(1S,3R,4R,6S)-1,3,4,6-TETRAPKISPHOSPHATE | C6 H16 O18 P4 | 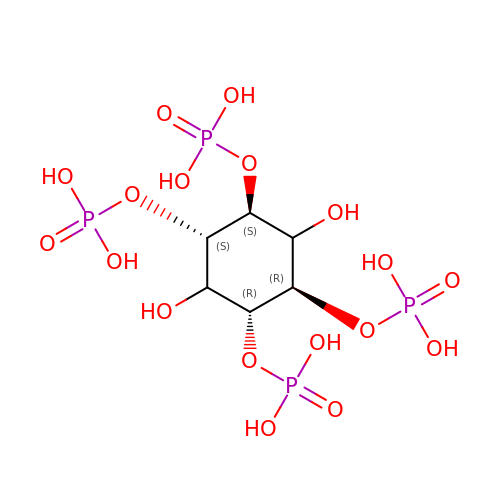ZAWIXNGTTZTBKV-JMVOWJSSSA-N>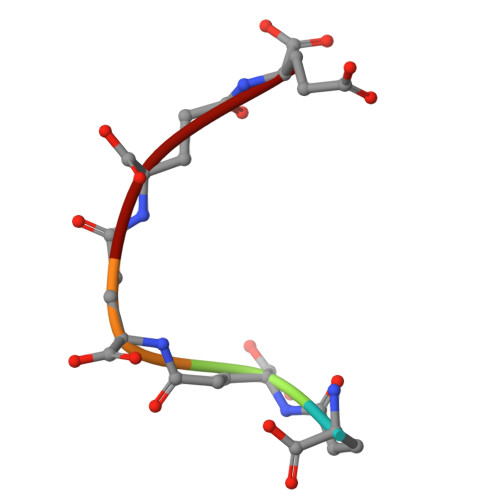 EEEEE> CQL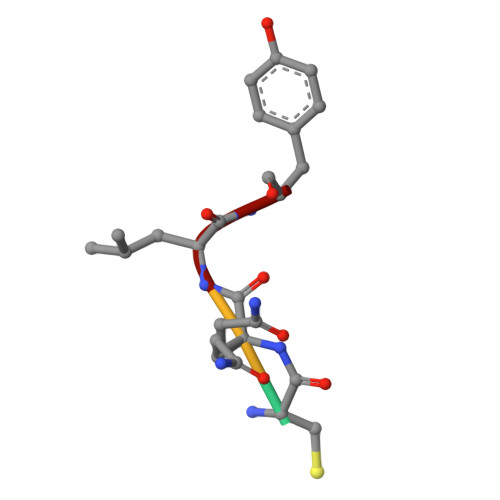Y> GSTGSPPGPPEDVTIDEITDTTAQLSWRPGADNHSPITMYVVQARTPFSVGWQAVSTVPEVIDGKTFTATVVGLNPWVEYEFRVVAANLIGIGEPSRPSENRRTEEALPEVTPANVSGGGGSKSELVITWETVPEELQNGGGFGYVVAFRPFGTISWMQAAVASPDASRYVFRNESLPPFSPYEVKVGVANNKGAGSFSPVTVVYSAEEEPTRAPITVLARSLSATDIEISWAPPRENQHKGRIQGYEVRCWRHDEKEENARKIRTVGNQTSAKVTNLQGNALYHLAVKAYNTAGTGPSSAMVNVTTKK

Contactins (CNTNs) are neural cell adhesion molecules that encode axon-target specificity during the patterning of the vertebrate visual and olfactory systems. Because CNTNs are tethered to the plasma membrane by a glycosylphosphatidylinositol anchor, they lack an intracellular region to communicate across the membrane. Instead, they form coreceptor complexes with distinct transmembrane proteins to transmit signals inside the cell. Finally, structural analyses of five CNTN–amyloid pairs indicate that these proteins interact through a conserved interface involving the second fibronectin type III repeat of CNTNs and the copper-binding domain of amyloid proteins.

We designed three variants of chicken CNTN4 by changing interface residues to alanine to validate our structural results. Residues T751/V752 or Y781/E786 were substituted with alanine in the first two mutants, whereas all four residues were mutated to alanine in the third. Introducing alanine residues at positions 751 and 752 in CNTN4 resulted in a fourfold-reduced affinity for APP. Residues Y781 and E786 interact with H137 in APP, and changing these two residues to alanine led to a 20-fold weaker binding (KD = 115 μM versus 5.4 μM). Finally, introducing alanine residues at positions T751, V752, Y781, and E786 results in a protein that does not bind to immobilized APP. Importantly, this difference in binding affinity is not because of any gross structural change brought about by the introduction of alanine residues as evidenced by comparing the structure of chicken CNTN4 with a mutant that includes all four alanine mutations. Consistent with these crystallographic results, mutations of residues T751, V752, Y781, and E786 to alanine in chicken CNTN4 that prevented binding to CNTN4 also abolished its binding to APLP2. Overall, these binding analyses indicate that the interface identified between the FN2 of CNTN4 and the copper-binding region of APP represents likely the arrangement of these two receptors on the surface of cells.(8M)-8-(2,3-dihydro-1,4-benzodioxin-6-yl)-2-(morpholin-4-yl)-4H-1-benzopyran-4-one 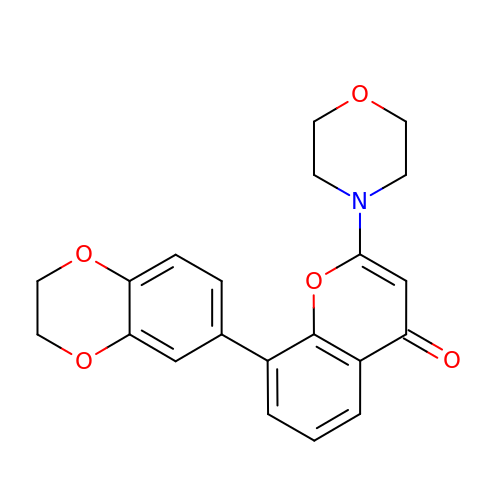| C21 H19 N O5 | PZGGPBWCQBEFPX-UHFFFAOYSA-N>[4x]NEQLAKQKGCMACHDLKAKKVGPAYADVAKKY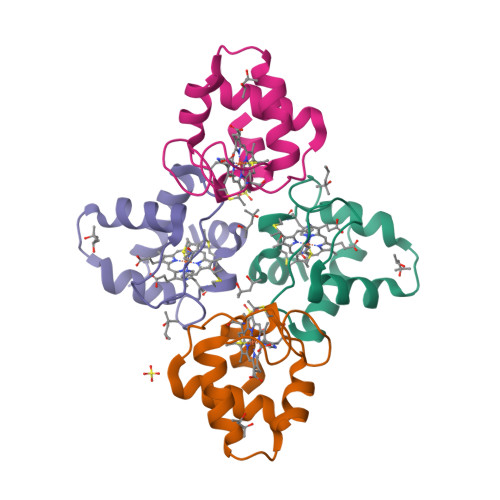AGRKDAVDYLAGKIKKGGSGVWGSVPMPPQNVTDAEAKQLAQWILSIK> SNAMNITLLKSKIHRASVTEARL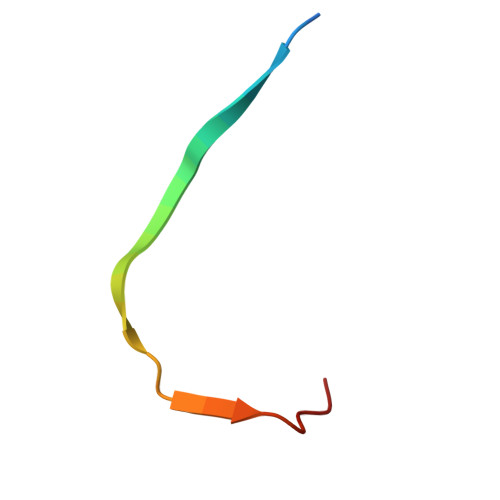DYIG> GAMEMLPNQTIYINNLNEKIKKEELKKSLYAIFSQ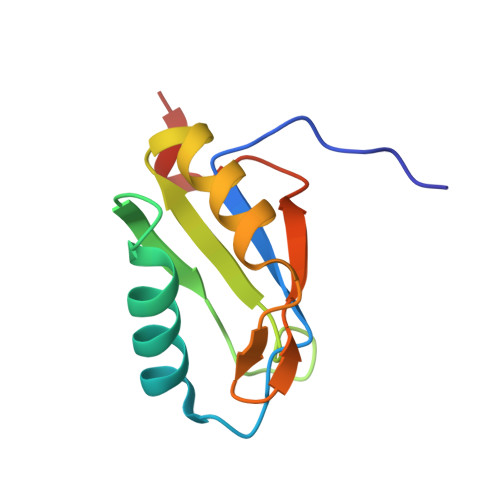FGQILDIVALKTLKMRGQAFVIFKEIGSASNALRTMQGFPFYDKPMQIAYSKSDSDIVAKIKG>SNAPRGGKVLDTSVLVDGRVAEVAAVGFLEGPLWVPHFVLKELQHFADSQDP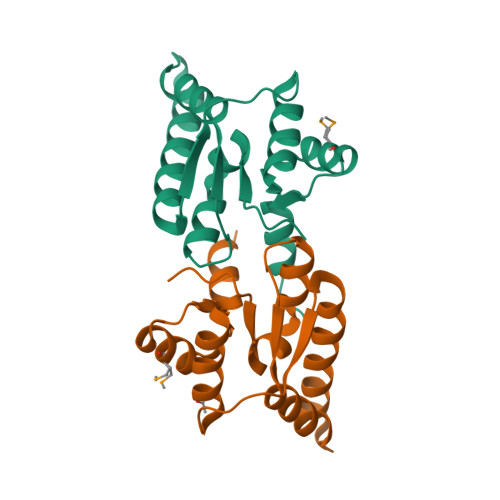LRRAKGRRGLETLERLREAAPLEVLETTPKGESVDEKLLFLARDLEAALVTNDHALLQMARIYGVKALSIQALAQALRPQLQ[2x]>GPMGNFIITERKKAKEER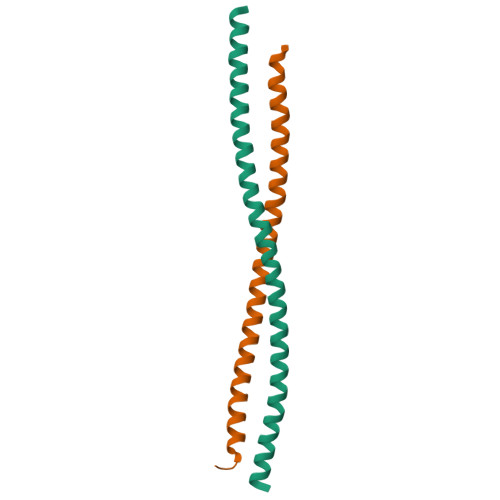SNPQTDSMDDLLIRRLTDRNDKEAHLNELFQDNSGAIGGNIVSHDDALLNTLAILQKELKSKEQEIRRLKEVIALKNKNTERLNAALISGTIENNVLQQKLSDLKKEHSQLVARWLKKTEKETEAMNSEIDGTK[2x]>[3x]MKFKHQGLVADLLPNIRVMQGVGHFMFNYYSEGKKFPHRIYCIVTLLLLLLQYGMMAVNLMMESDDVDDLTANTITMLFFLHPIVKMIYFPVRSKIFYKTLAIWNNPNSHPLFAESNARFHALAITKMRRLLFCVAGATIFSVISWTGITFIEDSVKRITDPETNETTIIPIPRLMIRTFYPFNAMSGAGHVFALIYQFYYLVISMAVSNSLDVLFCSWLLFACEQLQHLKAIMKPLMELSATLDTVVPNSGELFKAGSADHLRESQGVQPSGNGDNVLDVDLRGIYSNRQDFTATFRPTAGTTFNGGVGPNGLTKKQEMLVRSAIKYWVERHKHVVRLVTAVGDAYGVALLLHMLTTTITLTLLAYQATKVNGVNVYAATVIGYLLYTLGQVFLFC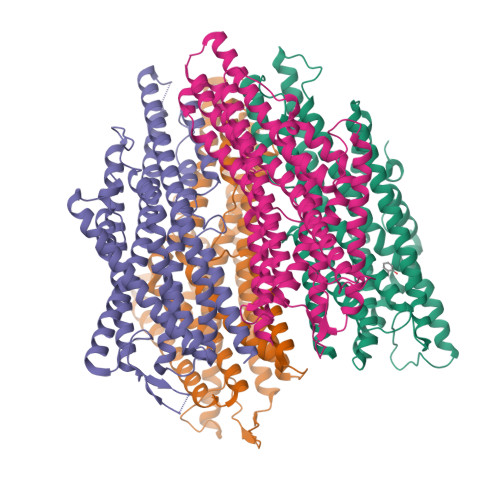IFGNRLIEESSSVMEAAYSCHWYDGSEEAKTFVQIVCQQCQKAMSISGAKFFTVSLDLFASVLGAVVTYFMVLVQLK;> MASILDCPIVSVNARVWRFWSFVLKHDAMRYISIIPVTVMTFFMFTDLCRSWGNIQELIIKAYFAVLYFNAVLRTLILVKDRKLYENFMQGISNVYFEISHIDDHKIQSLLKSYTVRARMLSISNLALGAIISTCFVVYPIFTGERGLPYGMFIPGLDSFRSPHYEIIYIVQVVLTFPGCCMYIPFTSFFASTTLFGLVQIKTLQRQLQTFKDNINSQDKEKVKAKVVKLIEDHKRIITYVSELNSLVTYICFVEFLSFGMMLCALLFLLNVIENHAQIVIVAAYIFMIISQIFAFYWHANEVREESMNLAEAAYSGPWVELDNSIKKKLLLIILRAQQPLEITVGNVYPMTLEMFQSLLNASYSYFTLLRRVYN>ACGLVASNLNAKPGECLKVRGELAPDAKSFVLNLGKDSNNLCLHFNPRFNAHGDANTIVCNSKDDGTWGTEQRETAFPFQPGSITEVCITFDQADLTIKLPDGHEFKFPNRLNMEAINYM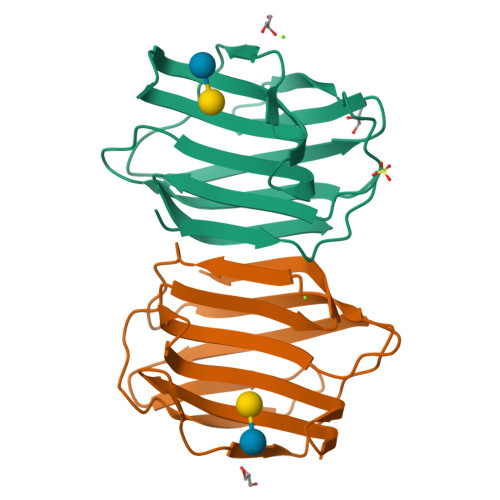AADGDFKIKCVAFE[6x]> KKPGVGTYATVDKLKAFDVTDGKKDAFTIKDTVRLYNVEEGKTYAIAGQLYEQSVAGDEGSALAKAATTVKVTASMAKPATEVEKTKYGEDVKVYETEMDLTVKREDLTKNQVVKDDIALVVYEQLWAEGTYEKVNDTEVTPKGKSEPVAKH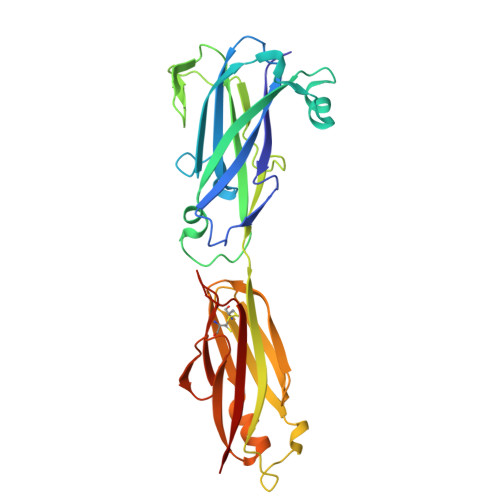NDPQSSSQSITAEPQFGSLKLTKTVTGWEDAFAKVARPEASYKFTVKCVQKGSVDEFTLKEGEEKTVEGIPLGDTCTISEDVQGAVNQAGLKDTVKFTAVNGVTVDSQVNGEAVVKIGGTANGSDTVANVEVTAENSFSY>MVTRIVILGGGPAGYEAALVAATSHPETTQVTVIDCDGIGGAAVLDDCVPSKTFIASTGLRTELRRAPHLGFHIDFDDAKISLPQIHARVKTLAAAQSADITAQLLSMGVQVIAGRGELIDSTPGLARHRIKATAADGSTSEHEADVVLVATGASPRILPSAQPDGERILTWRQLYDLDALPDHLIVVGSGVTGAEFVDAYTELGVPVTVVASQDHVLPYEDADAALVLEESFAERGVRLFKNARAASVTRTGAGVLVTMTDGRTVEGSHALMTIGSVPNTSGLGLERVGIQLGRGNYLTVDRVSRTLATGIYAAGDCTGLLPLASVAAMQGRIAMYHALGEGVSPIRLRTVAATVFTRPEIAAVGVPQSVIDAGSVAARTIMLPLRTNARAKMSEMRHGFVKIFCRRSTGVVIGGVVVAPIASEL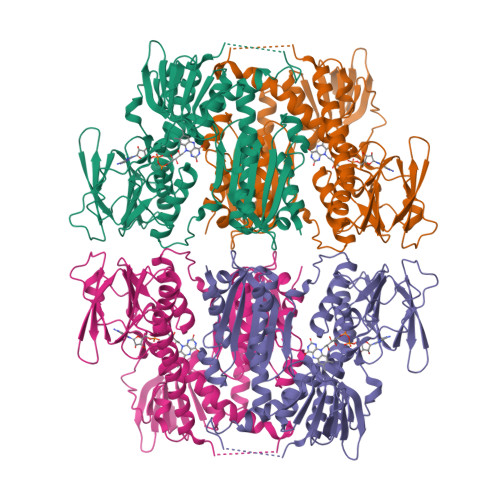ILPIAVAVQNRITVNELAQTLAVYPSLSGSITEAARRLMAHDDLDCTAAQDAAEQLALVPHHLPTSNHHHHHH[2x]> MQGPSFPEPKVVRSQGGLLSLKLSATPTPLALAGQRATLLTYGGSFPGPTLRVRPRDTVRLTLENRLPEPTNLHWHGLPISPKVDDPFLEIPPGESWTYEFTVPKELAGTFWYHPHLHGRVAPQLFAGLLGALVVESSLDAIPELREAEEHLLVLKDLALQGGRPAPHTPMDWMNGKEGDLVLVNGALRPTLVAQKATLRLRLLNASNARYYRLALQDHPLYLIAADGGFLEEPLEVSELLLAPGERAEVLVRLRKEGRFLLQALPYDRGAMGGMPQGPSRPETLLYLIAPKNPKPLPLPKALSPFPTLPAPVVTRRLVLTEDMMAARFFINGQVFDHRRVDLKGQAQTVEVWEVENQGDMDHPFHLHVHPFQVLSVGGRPFPYRAWKDVVNLKAGEVARLLVPLREKGRTVFHCHIVEHEDRGMMGVLEVG

Laccases are enzymes that belong to the family of multicopper oxidases (MCOs) and catalyze the oxidation of a phenolic and non-phenolic substrate to the reduction of a molecule of oxygen to form two water molecules. These enzymes have four catalytic coppers, a type 1 copper (CuT1), close to the surface, and a trinuclear center (TNC) formed by one type 2 copper (CuT2) and two type 3 coppers (CuT3). The Tth-Lac is the only laccase that presents a β-hairpin (Ala292–Gln307) close to the substrate binding site and the CuT1 site. The hairpin comprises two antiparallel β-strands (β22 and β23) and a connecting loop of six residues.

The deletion of P1Tth-Lac extends from Met295 to His303 with an additional A304G mutation. The protein crystal from the P1Tth-Lac mutant laccase is distinct from those reported for wild-type Tth-Laccase. The final model at 1.6 Å resolution shows acceptable refinement and stereochemical statistics. The majority of mainchain atoms have close superposition with the greatest deviation localized to residues M293 to P312. The region with the most structural discrepancy corresponds to the sequence (G304-P312) immediately downstream of the nine deleted residues of the β-hairpin (M295-H303). As would be expected, the shortening of the β-hairpin sequence resulted in the loss of antiparallel beta-strands and the flexible β-loop that covers the substrate channel. It appears to have destabilized these residues (Q307, G308, P309, S310) and their polar contacts normally present in Tth-Lac. Higher B-factors of the residues downstream of the deletion indicate increased flexibility (Q307, G308, P309, S310) that were otherwise more ordered in the Tth-Lac structure. P1Tth-Lac shows no significant changes in the residues that coordinate the CuT1 site (His393, Cys445, His450, and Met455), nor in the residues proposed to bind the ABTS substrate (Tyr288, Tyr232, Arg290, Met355, Asp390, Met 391, Met354, Lys424). It shows the coordination of all four Cu atoms by their coordinating residues, and they align well with the Tth-Lac structure, suggesting there was no disruption of the tertiary structure or the active center.The human pathogen Mycoplasma genitalium, a member of the pneumoniae cluster of mycoplasmas, binds to eukaryotic cells by means of its adhesion complex, the Nap. This complex is formed by two heterodimers, each consisting of proteins P110 and P1401–6. In addition to their roles in cytadherence and motility, P110 and P140 are immunodominant proteins and constitute the main target of host antibodies during infection. Here, we address the structure and mechanism of the Nap adhesion complex and reveal an intricate interplay between P110 and P140.

Crystals were obtained from the extracellular region of P140 (residues 23–1351), both alone and in complex with the N-terminal domain of P110 (P110N: residues 23–827). The structure of P140, for which there are no molecular models or experimental phases available, was determined by density modification techniques, starting with a mask derived from the sub-tomogram-averaged map of the whole Nap obtained by cryo-electron tomography (cryo-ET). The structure of the extracellular region of P140, with a bulky N-terminal domain (residues 23–1243) and a small C-terminal domain (residues 1244–1351), has an overall shape resembling the capital letter P. The N-terminal domain consists of a seven-bladed (β-sheet) propeller and a “crown” formed by the clustering of the long polypeptide segments that emerge from the propeller. β-Sheets I to VI each have four strands, while β-sheet VII, the last β-sheet in the propeller that connects directly with the C-terminal domain, has only two strands. P140 and P110 share many features of domain organization and the topology of the secondary structural elements, suggesting a common ancestor, although the degree of conservation differs for the N-terminal and C-terminal domains. The N-terminal domains, with an RMSD of 3.5 Å between the Cα atoms of 359 structurally equivalent residues (∼28%), are markedly different in the crown. In contrast, the C-terminal domains are closely related, with 74 equivalent residues (∼71%) and an RMSD of 2.2 Å.

>[6x]SVKHQQAVDETLTPWTWNNNNFSSLKITGENPGSFGLVRSQNDNLNISSVTKNSSDDNLKYLNAVEKYLDGQQNFAIRRYDNNGRALYDINLAKMENPSTVQRGLNGEPIFDPFKGFGLTGNAPTDWNEIKGKVPVEVVQSPHSPNLYFVLLVPKVALEYHNLNNQVVKESLEVKATQSSFNPTQRLQKDSPVKDSSKQGEKLSETTASSMSSGMATSTRAKALKVEVERGSQSDSLLKNDFAKKPLKHKNSSGEVKLEAEKEFTEAWKPLLTTDQIAREKGMGATVVSFYDAPYSENHTAFGLVDHIDPKKMVENYPPSWKTPKWNHHGIWDYNARNLLLQTTGFFNPRRHPEWFDEGQAKADNTSPGFKVGDTDHKKDGFKKNSSSPIALPFEAYFANIGNMVAIGNSVFIFGGNGHATKMFTTNPLSIGVFRIKYTDNFSKSSVTGWPYAVLFGGLINPQTNGLKDLPLGTNRWFEYVPRMAVSGVKWVGNQLVLAGTLTMGDTATVPRLKYDQLEKHLNLVAQGQGLLREDLQIFTPYGWANRPDIPVGAWLQDEMGSKFGPHYFLNNPDIQDNVNNDTVEALISSYKNTDKLKHVYPYRYSGLYAWQLFNWSNKLTNTPLSANFVNENSYAPNSLFAAILNEDLLTGLSDKIFYGKENEFAENEADRFNQLLSLNPNPNTNWARYLNVVQRFTTGPNLDSSTFDQFLDFLPWIGNGKPFSNSPSPSTSASSSTPLPTFSNINVGVKSMITQHLNKENTRWVFIPNFSPDIWTGAGYRVQSANQKNGIPFEQVKPSNNSTPFDPNSDDNKVTPSGGSSKPTTYPALPNSISPTSDWINALTFTNKNNPQRNQLLLRSLLGTIPVLINKSGDSNDQFNKDSEQKWDKTETNEGNLPGFGEVNGLYNAALLHTYGFFGTNTNSTDPKIGFKADSSSSSSSTLVGSGLNWTSQDVGNLVVINDTSFGFQLGGWFITFTDFIRPRTGYLGITLSSLQDQTIIWADQPWTSFKGSYLDSDGTPKSLWDPTALKSLPNSSTTYDTNPTLSPSFQLYQPNKVKAYQTTNTYNKLIEPVDATSAATNMTSLLKLLTTKNIKAKLGKGTASSQGNNNGGGVSQTINTITTTGNISEGLKEETSIQAETLKKFFDSKQNNKSEIGIGDSTFTKMDGKLTGVVSTPLVNLINGQGATSDSDTEKISFKPGNQIDFNRLFTLPVTELFDPNTMFVYDQYVPLLVNLPSGFDQASIRLKVISYSVENQTLGVRLEFKDPQTQQFIPVLNASSTGPQTVFQPFNQWADHHHHHH Nitrogenase provides access to bioessential nitrogen via the reduction of highly inert atmospheric dinitrogen (N2) to ammonia (NH3). In all nitrogenase isozymes, H-subunits form a homodimeric reductase component (‘HH’) that transiently associates with and transfers electrons to a catalytic core. This catalytic component is a heterotetramer composed of two D- and two K-subunits (‘DDKK’ or α2β2) and contains the active site metallocluster where N2 is bound and reduced to NH3. Three previously characterized ancestral variants were targeted from phylogenetic nodes within the evolutionary lineage of Azotobacter vinelandii Nif (wild-type, ‘WT’) (Garcia et al., 2023): Anc1A, Anc1B, and Anc2.

Anc1A and Anc1B are the same age, whereas Anc2 is reconstructed from an older phylogenetic node. As an additional distinction, Anc1A and Anc2 contain an ancestral D-subunit protein complexed with WT H- and K-subunit proteins. Specifically, all ancestors crystallized at pH 6.5, which is unusually acidic for nitrogenase. In addition, all ancestral proteins crystallized in space group P 212121, which differs from the space groups for the same proteins in A. vinelandii NifDK (i.e., WT; space group P 21), Clostridium pasteurianum Nif (space group P 21), and Klebsiella pneumoniae NifDK (space group C 2). All three ancestors showed anisotropic diffraction: 2.65–2.93 Å for Anc1A, 1.82–2.8 Å for Anc1B, and 1.82–2.42 Å for Anc2. Global structural differences between the ancestors and WT A. vinelandii DDKK are relatively minor and within the range of variation for available extant structures. Among the two hybrid ancestors, the RMSD between Anc2 and WT (0.24 Å) is smaller than that between Anc1A and WT (0.31 Å). Notably, a non-conserved Nif-D α-helix (positions 165–174 in Anc1B) lies within interacting distance of HH. This helix contains several substitutions across all ancestors, albeit the positioning of polar amino acids differs among Anc1A, Anc1B, and Anc2. Herein, the D-subunit S165A substitution is consistently present across all ancestors and may influence interactions with HH S175 in the ATP-bound complex, potentially reducing stability.

>[2x]MSTASWSHPQFEKMTREETQALIQEVLEVYPEKARKDRAKHLAVNDPSIEQSKKCITSNRKSLPGVMTVRGCAYAGSKGVVWGPIKDMIHISHGPVGCGQYSRAGRRNYYTGTTGVNTFGTMNFTSDFQEKDIVFGGDKKLAKIIDEIETLFPLNKGISVQSECPIGLIGDDIEAVAKKASKEIGKPVVPVRCEGFRGVSQSLGHHIANDAIRDWVLDKRDGQSFESTPYDVAIIGDYNIGGDAWSSRILLEEMGLRVVAQWSGDGTLAEMENTPKVKLNLLHCYRSMNYISRHMEEKYGIPWMEYNFFGPTKIAESLRKIAAHFDDTIQENAERVIAKYQPMMEAVIAKYRPRLEGKKVMLYVGGLRPRHVIGAYEDLGMEVVGTGYEFAHNDDYDRTIKELGDATLLYDDVTGYELEEFVKRLKPDLIGSGIKEKYIFQKMGIPFRQMHSWDYSGPYHGYDGFAIFARDMDMTLNNPCWNKLTPPWKKT;>MSQQVDKIKASYPLFLDQDYKDMLAKKRDGFEEKYPQDKIDEVFQWTTTKEYQELNFQREALTVNPAKACQPLGAVLCALGFEKTMPYVHGSQGCVAYFRSYFNRHFREPVSCVSDSMTEDAAVFGGQQNMKDGLQNCKATYKPDMIAVSTTCMAEVIGDDLNAFINNSKKEGFIPDEFPVPFAHTPSFVGSHVTGWDNMFEGIARYFTLKSMDDKVVGSNKKINIVPGFETYLGNFRVIKRMLSEMGVGYSLLSDPEEVLDTPADGQFRMYAGGTTQEEMKDAPNALNTVLLQPWHLEKTKKFVEGTWKHEVPKLNIPMGLDWTDEFLMKVSEISGQPIPASLTKERGRLVDMMTDSHTWLHGKRFALWGDPDFVMGLVKFLLELGCEPVHILCHNGNKRWKKAVDAILAASPYGKNATVYIGKDLWHLRSLVFTDKPDFMIGNSYGKFIQRDTLHKGKEFEVPLIRIGFPIFDRHHLHRSTTLGYEGAMQILTTLVNSILERLDEETRGMQATDYNHDLVR[2x]>[2x]MSLSTRIAPHLPYLRRFARSVTGSQSSGDAYVSAMLEALVADISIFPRASCDRIGTYWLFCHLFDQTTPNIPEPLPQFGLEQKTSAKLSYLTPRARQAFLLIAVEGFNEQEASEIMNLDARDFRKLLNQASIDISQQIATQV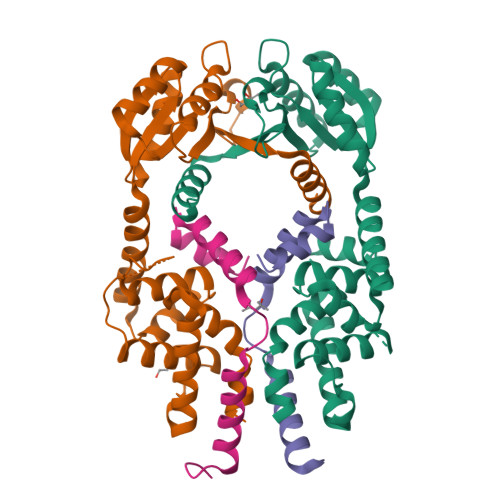MIIEDEPLIAMDIEQMVESLGHQVVGIARTRKEAVVMYHQKKPRLILADIQLADNSSGIDAVNDILQNDRIPVIFITAFPERLLTGERPEPTFLVTKPFNPDMVKALISQALFFKENASKAALEAGWSHPQFEK;>[2x]MGSSHHHHHHSQDPMNDCDEKNLTNHFTFGDDLLGVNSEIARKLRQFYLEIQEEALPARLLELLERLEQAERFGLNNAEKV ethyl 2-(naphthalen-2-ylamino)-4-oxidanylidene-furan-3-carboxylate 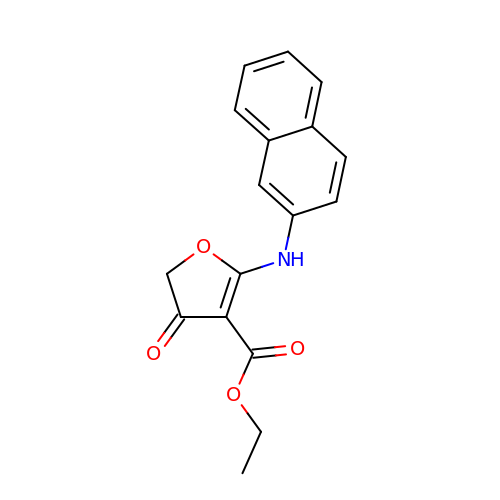| C17 H15 N O4 | KDQAZKWASGPNFD-UHFFFAOYSA-N>MTPPHNYLAVIKVVGIGGGGVNAVNRMIEQGLKGVEFIAINTDAQALLMSDADVKLDVGRDSTRGLGAGADPEVGRKAAEDAKDEIEELLRGADMVFVTAGE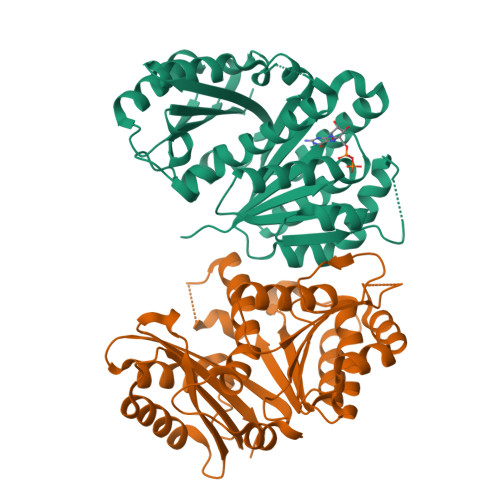GGGTGTGGAPVVASIARKLGALTVGVVTRPFSFEGKRRSNQAENGIAALRESCDTLIVIPNDRLLQMGDAAVSLMDAFRSADEVLLNGVQGITDLITTPGLINVDFADVKGIMSGAGTALMGIGSARGEGRSLKAAEIAINSPLLEASMEGAQGVLMSIAGGSDLGLFEINEAASLVQDAAHPDANIIFGTVIDDSLGDEVRVTVIAAGFD[2x]>[4x]MS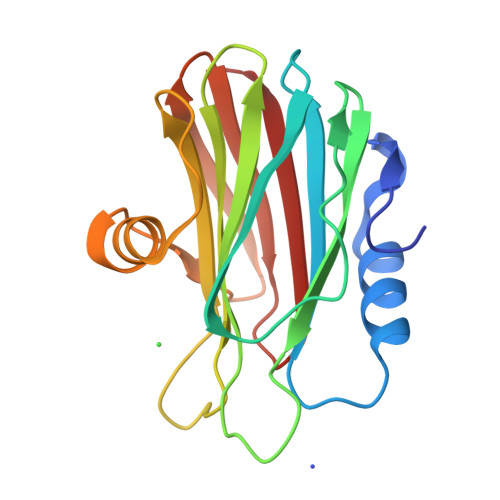ADVAGAVIDGAGLGFDVLKTVLEALGNVKRKIAVGIDNESGKTWTAMNTYFRSGTSDIVLPHKVAHGKALLYNGQKNRGPVATGVVGVIAYSMSDGNTLAVLFSVPYDYNWYSNWWNVRVYKGQKRADQRMYEELYYHRSPFRGDNGWHSRGLGYGLKSRGFMNSSGHAILEIHVTKA>[2x]SMKAVMSQALKATFSGFKKEQRRLGIPKNPWLWSE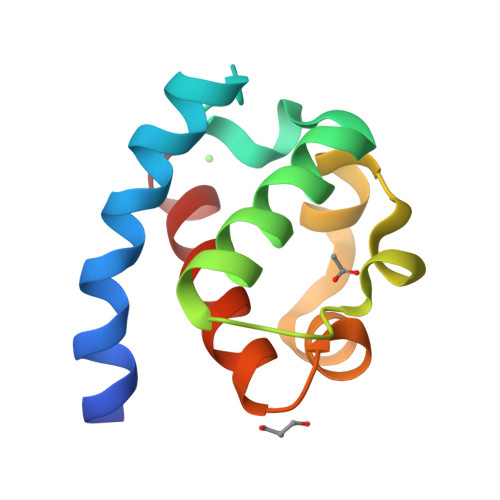QQVCQWLLWATNEFSLVNVNLQRFGMNGQMLCNLGKERFLELAPDFVGDILWEHLEQMIKEN> MNIKKEFIKVI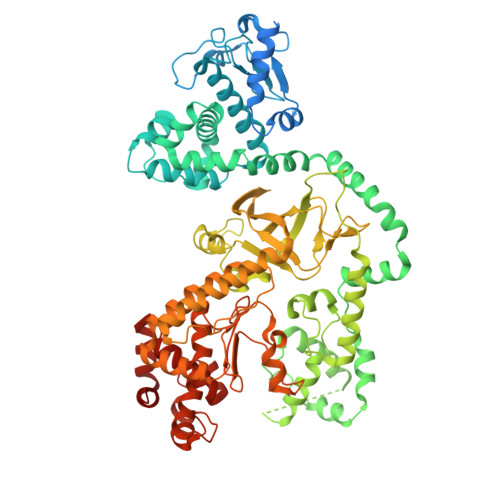SMSCLVTAITLSGPVFIPLVQGAGGHGDVGMHVKEKEKNKDENKRKDEERNKTQEEHLKEIMKHIVKIEVKGEEAVKKEAAEKLLEKVPSDVLEMYKAIGGKIYIVDGDITKHISLEALSEDKKKIKDIYGKDALLHEHYVYAKEGYEPVLVIQSSEDYVENTEKALNVYYEIGKILSRDILSKINQPYQKFLDVLNTIKNASDSDGQDLLFTNQLKEHPTDFSVEFLEQNSNEVQEVFAKAFAYYIEPQHRDVLQLYAPEAFNYMDKFNEQEINLSLEELKDQRMLARYEKWEKIKQHYQHWSDSLSEEGRGLLKKLQIPIEPKKDDIIHSLSQEEKELLKRIQIDSSDFLSTEEKEFLKKLQIDIRDSLSEEEKELLNRIQVDSSNPLSEKEKEFLKKLKLDIQPYDINQRLQDTGGLIDSPSINLDVRKQYKRDIQNIDALLHQSIGSTLYNKIYLYENMNINNLTATLGADLVDSTDNTKINRGIFNEFKKNFKYSISSNYMIVDINERPALDNERLKWRIQLSPDTRAGYLENGKLILQRNIGLEIKDVQIIKQSEKEYIRIDAKVVPKSKIDTKIQEAQLNINQEWNKALGLPKYTKLITFNVHNRYASNIVESAYLILNEWKNNIQSDLIKKVTNYLVDGNGRFVFTDITLPNIAEQYTHQDEIYEQVHSKGLYVPESRSILLHGPSKGVELRNDSEGFIHEFGHAVDDYAGYLLDKNQSDLVTNSKKFIDIFKEEGSNLTSYGRTNEAEFFAEAFRLMHSTDHAERLKVQKNAPKTFQFINDQIKFIINS>[2x]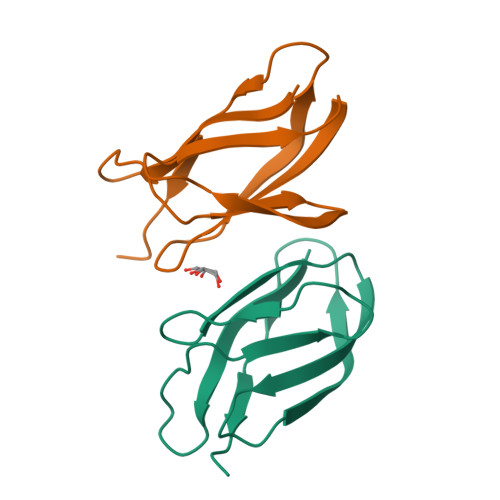SGVKGFVKDSITGSGLENATISVAGINHNITTGRFGDFYRLLVPGTYNLTVVLTGYMPLTVTNVVVKEGPATEVDFSLRPHH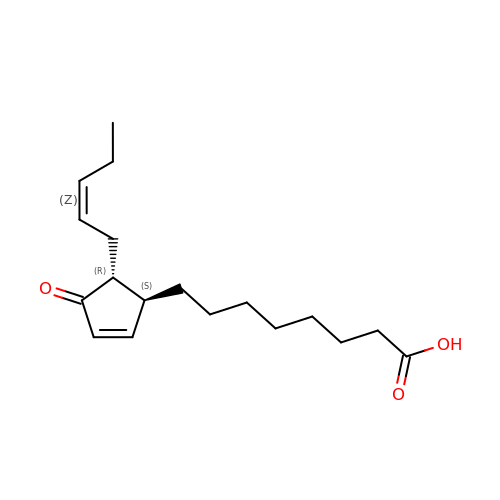9S,13R-12-OXOPHYTODIENOIC ACID | C18 H28 O3 | PMTMAFAPLCGXGK-TTXFDSJOSA-N>QNLGAAVAILGGPGTVQGVVRFLQLTPERCLIEGTIDGLEPGLHGLHVHQYGDLTNNCNSCGNHFNPDGASHGGPQDSDRHRGDLGNVRADADGRAIFRMEDEQ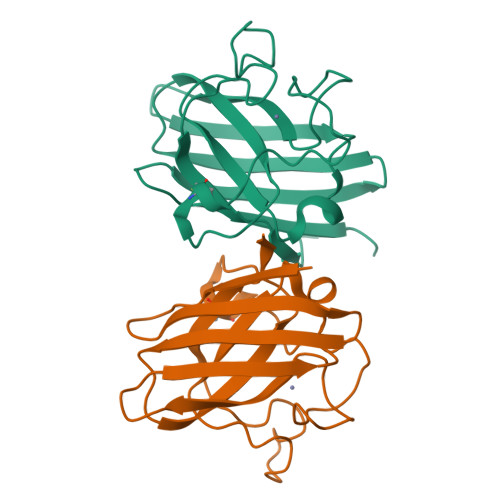LKVWDVIGRSLIIDEGEDDLGRGGHPLSKITGNSGERLACGIIARSAGLF[4x]The rational design of small molecules that target specific DNA sequences is a promising strategy to modulate gene expression. This report focuses on a diamidinobenzimidazole compound, whose selective binding to the minor groove of AT DNA sequences holds broad significance in the molecular recognition of AT-rich human promoter sequences. The specialized method of X-ray crystallography was utilized to investigate how the sequence-dependent recognition properties in general, A-tract, and alternating AT sequences affect the binding of diamidinobenzimidazole in the DNA minor groove. A strong and direct hydrogen bond between the N-H of the benzimidazole and an H-bond acceptor atom in the minor groove is essential for DNA recognition in all sequences described. In addition, the diamidine compound specifically utilizes an interfacial water molecule for its DNA binding.

We also describe the high-resolution X-ray structure of ATAT-DB1476 at 1.63 Å, with Rwork and Rfree at 18.3 and 20.1%, respectively. Like AAATTT-DB1476, the 1:1 complex structure of ATAT-DB1476 shows one favored orientation of the DB1476 model with strong direct hydrogen bonds at the −ATAT– minor groove. The specific and direct strong bifurcated hydrogen bonding between the B-N2 and O2 of T18 and T8, and the strong H-bond between C-N4 an O2 of C9 (3.0 Å) marked the DB1476 a strong ATAT (KD = 12 nM) binder. The bifurcated hydrogen bonding in the ATAT-DB1476 X-ray structure differs from the AATT-DB1476 structure in that N-H of the BI binds slightly further down the DNA (T7 in −AATT–, T8 in −ATAT−). ATAT-DB1476 shows an “external water” molecule. The unique external water stabilizes the ATAT-DB1476 complex structure by forming an H-bond with B-N1, confirming the singular DB1476 orientation at the −ATAT– minor groove. Due to the moderate flexibility and crescent-shaped DB1476, the direct strong H-bond at one amidine end (C-N4) allows the other end (A-N6) to form an indirect water-mediated H-bond with O2 of T20. Biosensor-SPR binding studies show that DB1476 binds ATAT about 10 times weaker than AATT. Yet DB1476 binding to the ATAT site is favored in one orientation in contrast to the AATT DNA. The selection of a particular orientation is not entirely understood, but we observe that the repeating symmetry units across the P212121 crystal lattice require an N6-BI-N4 orientation of DB1476 along the C1:G12 direction.

>CGCGATATCGCG[2x]>[2x]MSLKP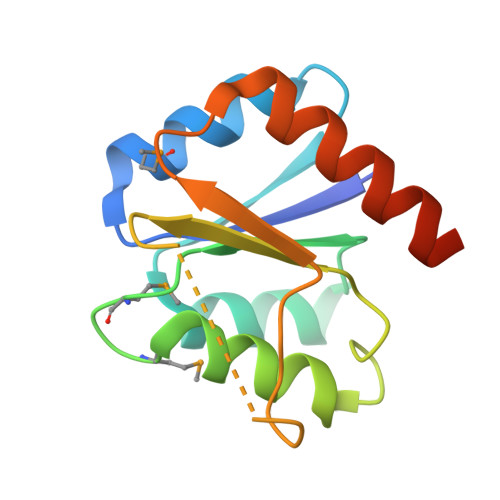KVLIVENSWTMRETLRLLLSGEFDCTTAADGASGLQQALAHPPDVLISDVNMDGMDGYALCGHFRSEPTLKHIPVIFVSGYAPRTEGPADQPVPDAYLVKPVKPPVLIAQLHALLARAEAEGHHHHHH>QTSCDQWATFTGNGYTVSNNLWGAS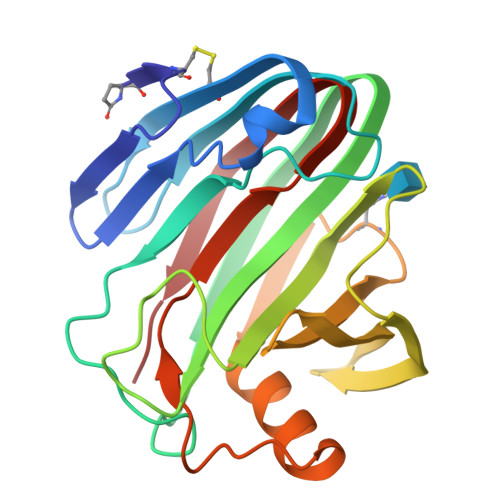AGSGFGCVTAVSLSGGASWHADWQWSGGQNNVKSYQNSQIAIPQKRTVNSISSMPTTASWSYSGSNIRANVAYDLFTAANPNHVTYSGDYELMIWLGKYGDIGPIGSSQGTVNVGGQSWTLYYGYNGAMQVYSFVAQTNTTNYSGDVKNFFNYLRDNKGYNAAGQYVLSYQFGTEPFTGSGTLNVASWTASIN[6x]>TQFD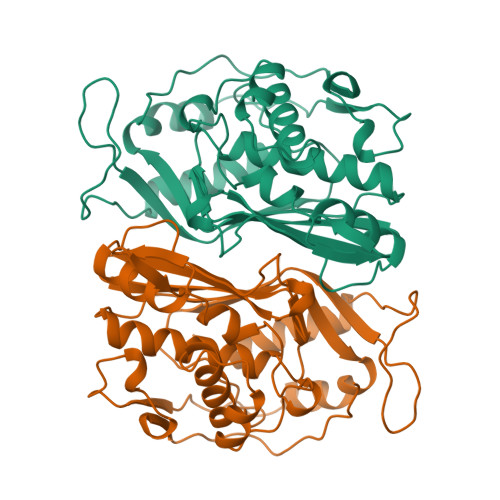KQYNSIIKDIINNGISDEEFDVRTKWDSDGTPAHTLSVISKQMRFDNSEVPILTTKKVAWKTAIKELLWIWQLKSNDVNDLNMMGVHIWDQWKQEDGTIGHAYGFQLGKKNRSLNGEKVDQVDYLLHQLKNNPSSRRHITMLWNPDELDAMALTPCVYETQWYVKHGKLHLEVRARSNDMALGNPFNVFQYNVLQRMIAQVTGYELGEYIFNIGDCHVYTRHIDNLKIQMEREQFEAPELWINPEVKDFYDFTIDDFKLINYKHGDKLLFEVAV[2x]> MEKATKRNDEECEVQLNIKRNSKHSAWTGELFKIECPVKYCVHRPNVTWCKHNGTIWVP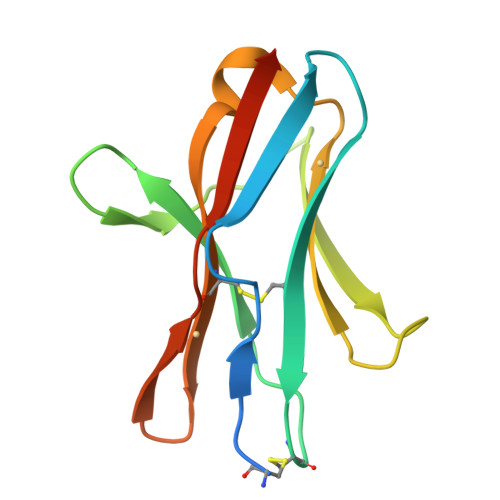LEVGPQLYTSWEENRSVPVFVLHFKPIHLSDNGSYSCSTNFNSQVINSHSVTIHVRERSQNSS> MEPAGRFTKVAAAVADSVVTIESVSDQEGMQGSGVIVDGRGYIVTNNHVISEAANNPSQFKTTVVFNDGKEVPANLVGRDPKTDLAVLKVDNVDNLTVARLGDSSKVRVGDEVLAVGAPLGLRSTVTQGIVSALHR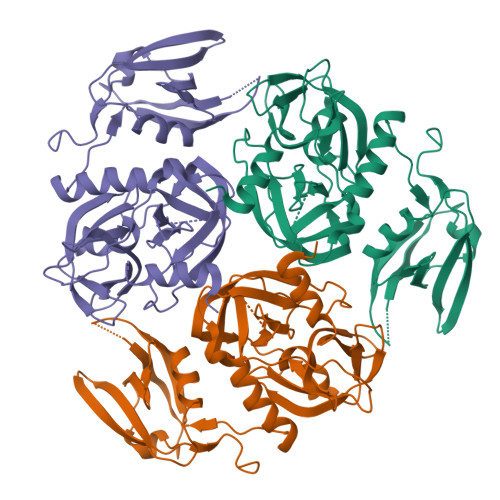PVPLSGEGSDTDTVIDAIQTDASINHGNSGGPLIDMDAQVIGINTAGKSLSDSASGLGFAIPVNEMKLVANSLIKDGAIVHPTLGISTRSVSNAIASGAQVANVKAGSPAQKGGILENDVIVKVGNRAVADSDEFVVAVRQLAIGQDAPIEVVREGRHVTLTVKPDPDSTLEHHHHHH3-[(1-ethanoyl-5-methoxy-indol-3-yl)carbonylamino]-4-fluoranyl-5-(1-methylpyrazol-4-yl)benzoic 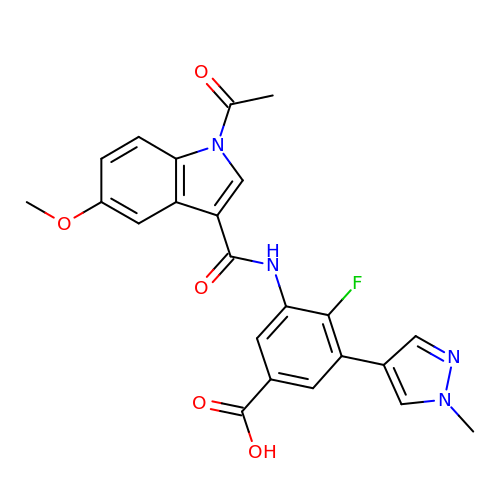acid | C23 H19 F N4 O5 | RCPJEOKKJODBRQ-UHFFFAOYSA-N>LDNGLLQTPPMGWLAWERFRCNINCDEDPKNCISEQLFMEMADRMAQDGWRDMGYTYLNIDDCWIGGRDASGRLMPDPKRFPHGIPFLADYVHSLGLKLGIYADMGNFTCMGYPGTTLDKVVQDAQTFAEWKVDMLKLDGCFSTPEERAQGYPKMAAALNATGRPIAFSCSWPAYEGGLPPRVQYSLLADICNLWRNYDDIQDSWWSVLSILNWFVEHQDILQPVAGPGHWNDPDMLLIGNFGLSLEQSRAQMALWTVLAAPLLMSTDLRTISAQN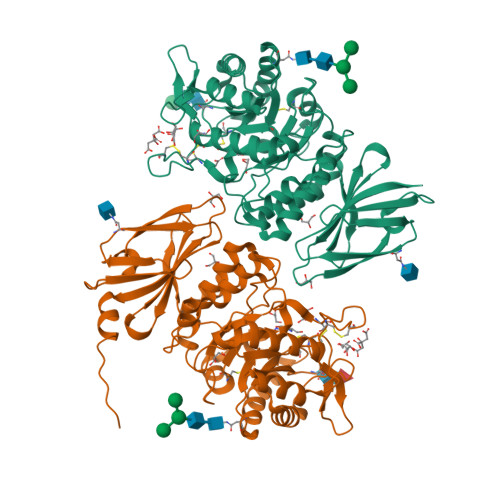MDILQNPLMIKINQDPLGIQGRRIHKEKSLIEVYMRPLSNKASALVFFSCRTDMPYRYHSSLGQLNFTGSVIYEAQDVYSGDIISGLRDETNFTVIINPSGVVMWYLYPIKNLEMSQQHHHHHH[2x]>TTTVGITLKDAVIMATERRVTMENFIMHKNGKKLFQIDTYTGMTIAGLVGDAQVLVRYMKAELELYRLQRRVNMPIEAVATLLSNMLNQVKYMPYMVQLLVGGIDTAPHVFSIDAAGGSVEDIYASTGSGSPFVYGVLESQYSEKMTVDEGVDLVIRAISAAKQRDSASGGMIDVAVITRKDGYVQLPTDQIESRIRKLGLIL[14x];>RAITVFSPDGRLFQVEYAREAVKKGSTALGMKFANGVLLISDKKVRSRLIEQNSIEKIQL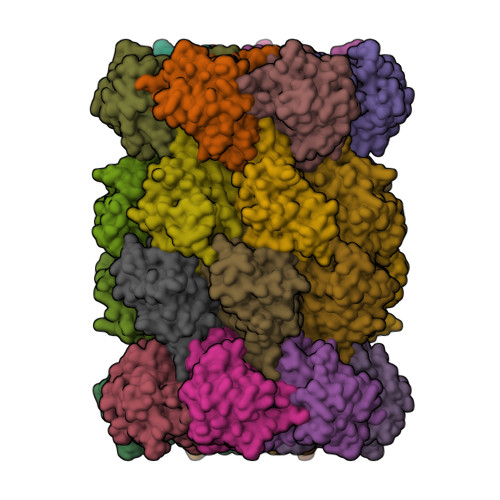IDDYVAAVTSGLVADARVLVDFARISAQQEKVTYGSLVNIENLVKRVADQMQQYTQYGGVRPYGVSLIFAGIDQIGPRLFDCDPAGTINEYKATAIGSGKDAVVSFLEREYKENLPEKEAVTLGIKALKSSLEEGEELKAPEIASITVGNKYRIYDQEEVKKFL[14x]> MTASSTGRTAIIAGNWKMNYGPREAAKFVQEIQPALSEALQAPGSPLCILCPPAISLAAVRAVLDIPDAASSAQIELGAQNMYFEEKGAFTGEISPNMVHELCTTVILGHSERRTYF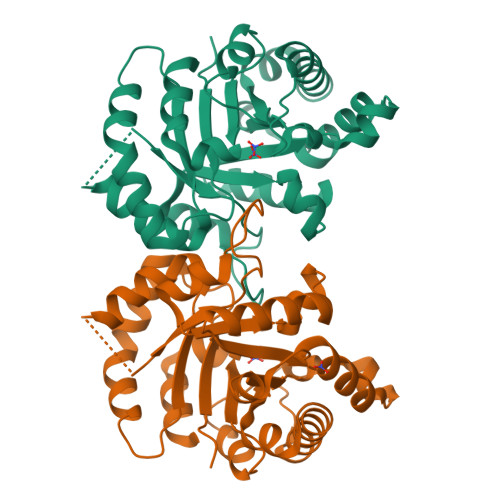GETDELVNKKTLAALRHELRPIVCIGENEQQHESGETAHIITTQVRASLANLTSEQAREIVIAYEPIWAIGTGKAATGEIANNVIRQIRQEYQAIYGAEAASVVRILYGGSVTSDNIAEFMAYPDIDGALVGGASLKPDFINIVRNSRQVRH>GAMADDAAIQQTLAKMGIKSSDIQPAPVAGMKTVLTNSGVLYITDDGKHIIQGPMYDVSGTAPVNVTNKMLLKQLNALEKEMIVYKAPQEKHVITVFTDITCGYSHKLHEQMADYNALGITVRYLAFPRQGLDSDAEKEMKAIWCAKDKNKAFDDVMAGKSVAPASCDVDIADHYALGVQLGVSGTPAVVLSNGTLVPGYQPPKEMKEFLDE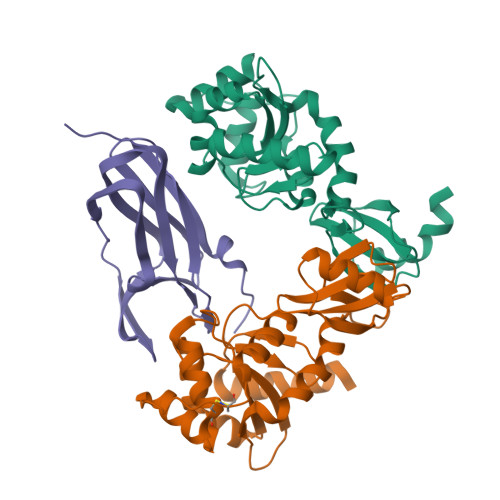HQKMTSGK[2x];> GLFDAPGRSQFVPADQAFAFDFQQNQHDLNLTWQIKDGYYLYRKQIRITPEHAKIADVQLPQGVWHEDEFYGKSEIYRDRLTLPVTINQASAGATLTVTYQGAADAGFCYPPETKTVPLSEVVANNAAPQPV> SLSCDASGVCDGRSRSFTSIPSGLTAAMKSLDLSFNKITYIGHGDLRACANLQVLILKSSRINTIEGDAFYSLGSLEHLDLSDNHLSSLSSSWFGPLSSLKYLNLMGNPYQTLGVTSLFPNLTNLQTLRIGNVETFSEIRRIDFAGLTSLNELEIKALSLRNYQSQSLKSIRDIHHLTLHLSESAFLLEIFADILSSVRYLELRDTNLARFQFSPLPVDEVSSPMKKLAFRGSVLTDESFNELLKLLRYILELSEVEFDDCTLNGLGDFNPSESDVVSELGKVETVTIRRLHIPQFYLFYDLSTVYSLLEKVKRITVENSKVFLVPCSFSQHLKSLEFLDLSENLMVEEYLKNSACKGAWPSLQTLVLSQNHLRSMQKTGEILLTLKNLTSLDISR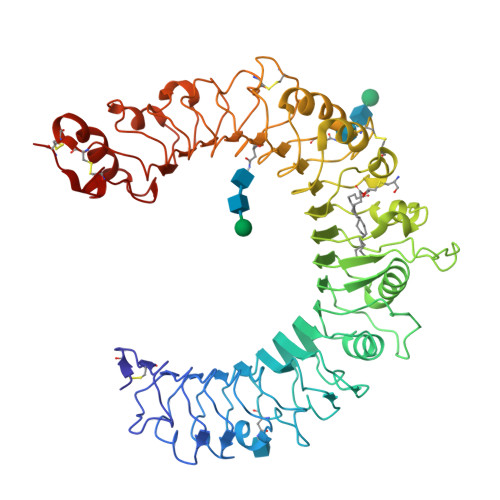NTFHPMPDSCQWPEKMRFLNLSSTGIRVVKTCIPQTLEVLDVSNNNLDSFSLFLPRLQELYISRNKLKTLPDASLFPVLLVMKISRNQLKSVPDGIFDRLTSLQKIWLHTNPWDCSCPRIDYLSRWLNKNSQKEQGSAKCSGSGKPVRSIICP[3-(3-{[2-chloro-3-(trifluoromethyl)benzyl](2,2-diphenylethyl)amino}propoxy)phenyl]acetic 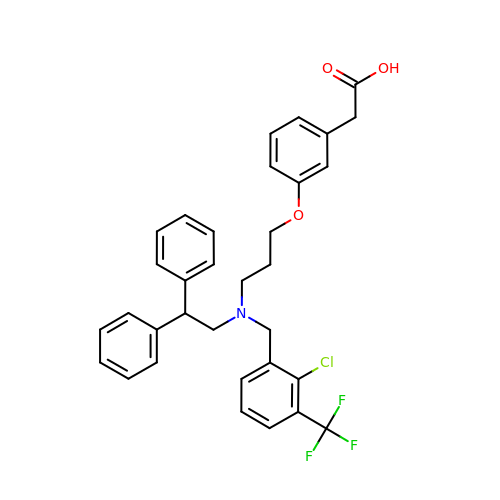acid | C33 H31 Cl F3 N O3 | NAXSRXHZFIBFMI-UHFFFAOYSA-N>TAAVALVKANENAAAILNLKNAIQKTNAAVADVVQATQSLGTAVQAVQDHINSVVSPAITAANY[2x];>QILSIDPLDISQNLAAVNKSLSDALQHLAQ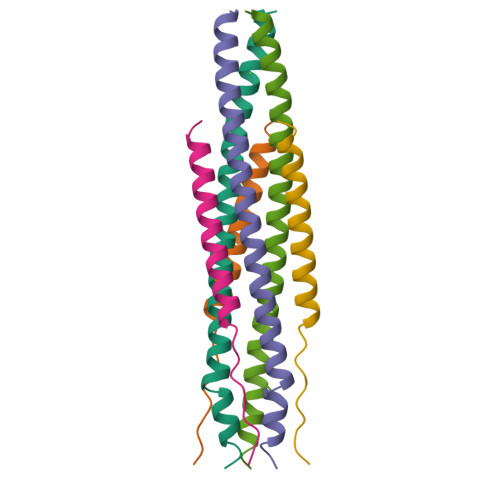SDTYLSAI[2x]>GPSRATMDTESQYSGYSYKSGHSRSSRKHRDRRDRHRSKSRDGGRGDKSVTIQAPGEPLLDNESTRGDERDDNWGETTTVVTGTSEHSISHDDLTRIAKDMEDSVPLDCSRHLGVAAGATLALLSFLTPLAFLLLPPLLWREELEPCGTACEGLFISVAFKLLILLLGSWALFFRRPKASLPRVFVLRALLMVLVFLLVVSYWLFYGVRILDARERSYQGVVQFAVSLVDALLFVHYLAVVLLELRQLQPQFTLKVVRSTDGASRFYNVGHLSIQRVAVWILEKYYHDFPVYNPALLNLPKSVLAKKVSGFKVYSLGEENSTNNSTGQSRAVIAAAARRRDNSHNEYYYEEAEHERRVRKRRARLVVAVEEAFTHIKRLQEEEQKNPREVMDPREAAQAIFASMARAMQK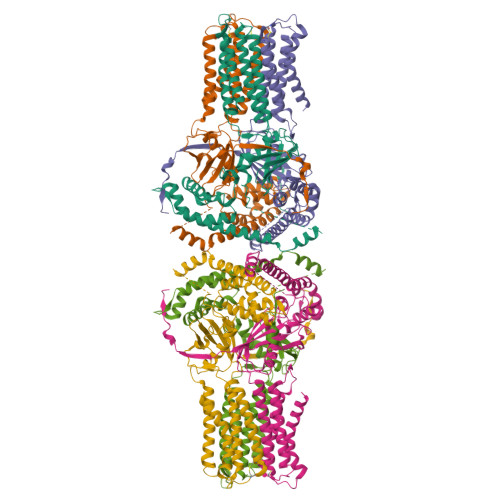YLRTTKQQPYHTMESILQHLEFCITHDMTPKAFLERYLAAGPTIQYHKERWLAKQWTLVSEEPVTNGLKDGIVFLLKRQDFSLVVSTKKVPFFKLSEEFVDPKSHKFVMRLQSETSV[6x]> MVKVGINGFGRIGRLVLRVCMEKGVRVVAVNDPFIDPEYMVYMFKYDSTHGRYKGTVEHKNGRLVVDNLEINVFQCKEPKEIPWSSVGNPYVVEATGVYLSIEAASGHISSGARRVIVTAPSPDAPMLVMGVNEKDYNPGSMTVVSNASCTTNCLAPLAKVIHERFGIVEGLMTTVHAYTATQKTVDGPSKKDWRGGRGAHQNIIPSSTGAAKAVGKVIPELNGKLTGMAFRVPTPNVSVVDLTCRL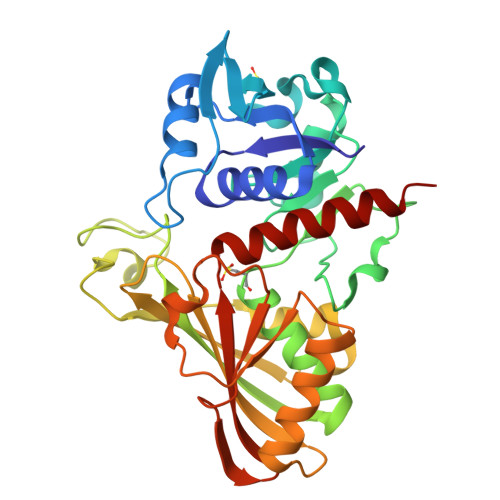AQPASYTAIKEAVKAAAKGPMAGILAYTEDQVVSTDFNGDSHSSIFDAKAGIALNDNFVKLVSWYDNEYGYSHRVVDLLRYMFSREK> ETKSYYQLPLMAQVGTQSTASQGNRLLWVEQVAVPDYLAGNGVVYQTSDVQYVIANNNLWASPLDQQLRNTLVANLSSQLPGWVVASQPLGSDQDTLNV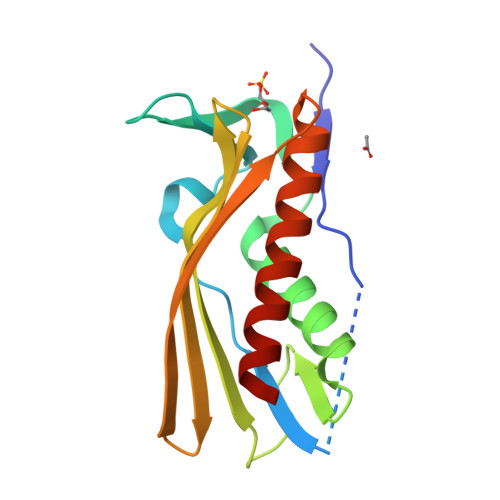TVTGFHGRYDGAVVISGEWLLNHQGQLIKRPFHLELKQQKDGYDEMVKVLAQGWAQESANIAREISRLP> MAQFPNTPSFTGFNTPSRIEADIADLAHEGTIPQGLNGAFYRVQPDPQFPPRLDDDIAFNGDGMITRFHIHDGQVDFRQRWAKTDKWKLENAAGKALFGAYRNPLTDDEAVKGEIRSTANTNAFVFGGKLWAMKEDSPALVMDPATMETFGFEKFGGKMTGQTFTAHPKVDPKTGNMVAIGYAASGLCTDDVTYMEVSPEGELVREVWFKVPYYCMMHDFGITEDYLVLHIVPSIGSWERLEQGKPHFGFDTTMPVHLGIIPRRDGVRQE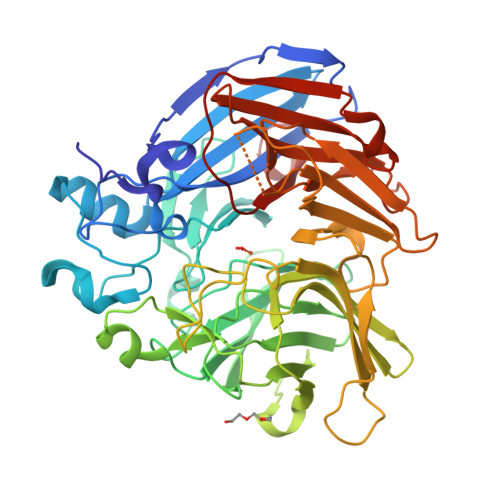DIRWFTRDNCFASHVLNAWQEGTKIHFVTCEAKNNMFPFFPDVHGAPFNGMEAMSHPTDWVVDMASNGEDFAGIVKLSDTAAEFPRIDDRFTGQKTRHGWFLEMDMKRPVELRGGSAGGLLMNCLFHKDFETGREQHWWCGPVSSLQEPCFVPRAKDAPEGDGWIVQVCNRLEEQRSDLLIFDALDIEKGPVATVNIPIRLRFGLHGNWANADEIGLAEKVLAA>[2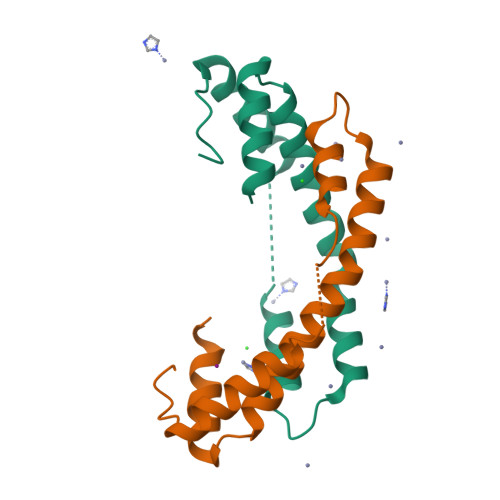x]SFKDLNLTDAQKQQIREIMKGQRDQMKRPPLEERRAMHDIIASDTFDKVKAEAQIAKMEEQRKANMLALMETQNKIYNILTPEQKKQFNANFEKRLT>[2x]APPPVPKTPAGPLTLSGQGSFFVGGRDVTSETLSLSPKYDAHGTVTVDQMYVRYQIPQRAKRYPITLIHGCCLTGMTWETTPDGRMGWDEYFLRKGYSTYVIDQSGRGRSATDISAINAVKLGKAPASSLPDLFAAGHEAAWAIFRFGPRYPDAFKDTQFPVQAQAELWQQMVPDWLGSMPTPNPTVANLSKLAIKLDGTVLLSHSQSGIYPFQTAAMN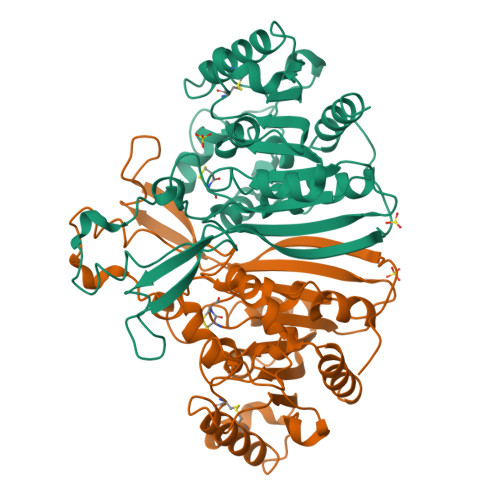PKGITAIVSVEPGECPKPEDVKPLTSIPVLVVFGDHIEEFPRWAPRLKACHAFIDALNAAGGKGQLMSLPALGVHGNSHMMMQDRNNLQVADLILDWIGRNTAKPAHGR>[2x]MKVTLSALDTSESSFTPLVVIELAQDVKEETKEWLKNRIIAKKKDGGAQLLFRPLLNKYEQETLENQNLYLVGASKIRMLLGAEAVGLVKECNDNTMRAFTYRTRQNFKGFDDNNDDFLTMAECQFIIKHELENLRAKDEKMIPGYPQAKLYPGKSLLRRLLTSGIVIQVFPLHDSEALKKLEDTWYTRFALKYQPIDSIRGYFGETIALYFGFLEYFTFALIPMAVIGLPYYLFVWEDYDKYVIFASFNLIWSTVILELWKRGCANMTYRWGTLLMKRKFEEPRPGFHGVLGINSITGKEEPLYPSYKRQLRIYLVSLPFVCLCLYFSLYVMMIYFDMEVWALGLHENSGSEWTSVLLYVPSIIYAIVIEIMNRLYRYAAEFLTSWENHRLESAYQNHLILKVLVFNFLNCFASLFYIAFVLKDMKLLRQSLATLLITSQILNQIMESFLPYWLQRKHGVRVKRKVQALKADIDATLYEQVILEKEMGTYLGTFDDYLELFLQ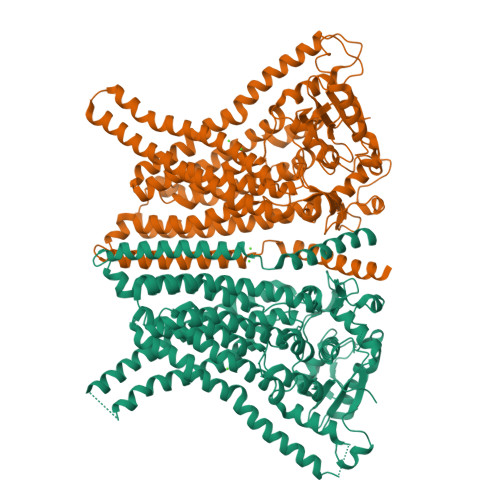FGYVSLFSCVYPLAAAFAVLNNFTEVNSDALKMCRVFKRPFSEPSANIGVWQLAFETMSVISVVTNCALIGMSPQVNAVFPESKADLILIVVAVEHALLALKFILAFAIPDKPRHIQMKLARLEFESLEALKQQQMKLVTENLKEEPMESGKEKATAENLYFQ> MAKEEVKQKKTKEKEPDITFF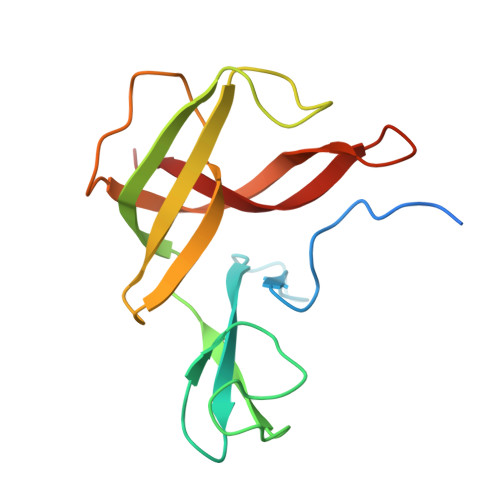HPDILEVPKDGGLPYLKGYRCKKCGQLDFKTEMCTNCWSEEFEMVPLSRRGKVYSFSDIYIGQQGLATPYIFAYVDLPENLRVFAQLEGEVDTYRCDEEVELTLGPIRMNNDNLPIISYKFKKIA>MSSFHLDDINWQPNIEGVYNSEQRFNLNDYFTSEKVPGDGNCFFYSVSFLLFESLSEWRSIKNTIASFAAANWGQCVQAKLNYAN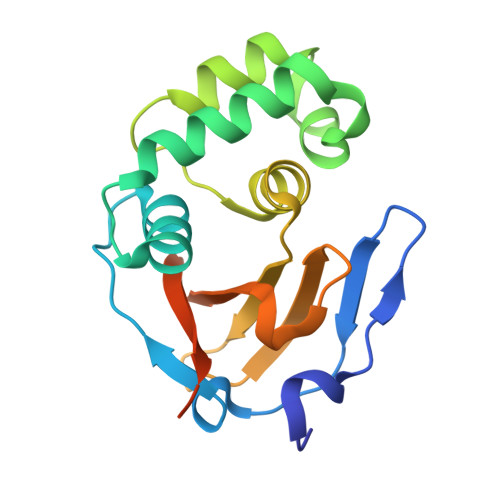SSDYRADMLRNYYWGGSVEAEILSKALNITIILWEADVSENVVTATKYGPGLVSTALNLKLCQGHIEPLQLMKLVDQDVLRKSGSHHHHHH[2x]> MTNESILESYSGVTPERKKSRMPAKLDWWQSATGLFLGLFMIGHMFFVSTILLGDNVMLWVTKKFELDFIFEGGKPIVVSFLAAFVFAVFIAHAFLAMRKFPINYRQYLTFKTHKDLMRHGDTTLWWIQAMTGFAMFFLGSVHLYIMMTQPQTIGPVSSSFRMVSEWMWPLYLVL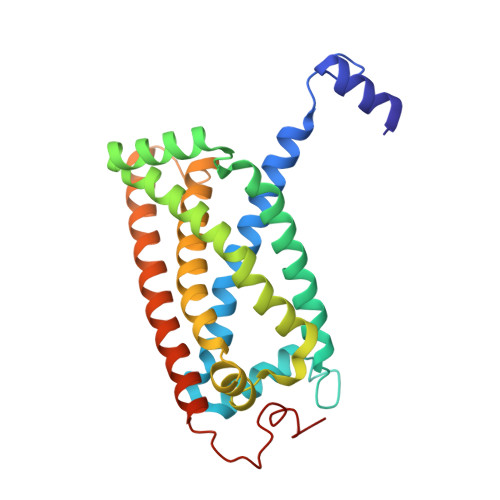LFAVELHGSVGLYRLAVKWGWFDGETPDKTRANLKKLKTLMSAFLIVLGLLTFGAYVKKGLEQTDPNIDYKYFDYKRTHEE>[4x]MDTPNKDDSIIRFSVSLQQNLLDELDNRIIKNGYSSRSELVRDMIREKLVEDNWAEDNPNDESKIAVLVVIYDHHQRELNQRMIDIQHASGTHVLSTTHIHMDEHNCLET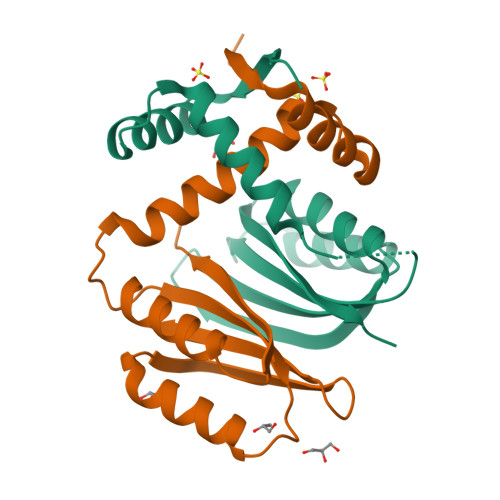IILQGNSFEIQRLQLEIGGLRGVKFAKLTKASSFEYNE>[2x]MNLKDSIGLRIKTERERQQMSREVLCLDGAELTVRQLIRIEKGESLPSLDRLSYIAKRLGKSMTELLDQDNITIPDEYYEMKNRLIKFPTYRNPDRIKSKLTLIEEVYEKFFDILPEEELLTLDILENILSFTSWEESPKVEEIYEDLFEQVKRKRKFSTNDLLVIDYYFFHLYGRKQYDKKLFERIIKRVLNQEIWTDDVYNIVLFNDLMAIAALKIFHNSFSDFLTVVDKALAVIEKSQLYSYKPSVFVLKAKYELLHKENKKEAAENYDKAIVFASVLEDSVLEESIKAGKLADGLGAGWSHPQFEK;>LPYFAGCL[2x]

Here, we elucidate the structure-function relationship of the transcription factor ComR, a new member of the RNPP family, which positively controls competence for natural DNA transformation in streptococci. ComR is directly activated by the binding of its associated pheromone XIP, the mature form of the comX/sigX-inducing-peptide ComS. XIP-binding induces release of the sequestered HTH domain and ComR dimerization to allow DNA binding. Each TPR domain is composed of 11 α-helices forming 5 TPR motifs followed by an additional C-terminal α-helix α16 called CAP.

The structure of the complex between full-length ComR from S. thermophilus LMD-9, the octapeptide XIP (ComS17-24 LPYFAGCL) and the pseudopalindromic 20 bp ComR-box from the comX promoter (5’-T10-A9-G8-T7-G6-A5-C4-A3-T2-A1.T1’-A2’-T3’-G4’-T5’-C6’-T7’-C8’-T9’-A10’-3’) has been determined at a resolution of 2.5 Å. The crystals diffracted in space group C2 with a dimer of the ComRS complex bound to one molecule of dsDNA per asymmetric unit. The two XRE-type HTH domains containing 5 α-helices (PROSITE documentation PDOC50943) interact with each other through loop α3-α4 and helix α5 whereas their two 32 Å-apart α3 helices perfectly accommodate in the successive DNA major groove of the two half-sites of the pseudopalindromic dsDNA fragment. H-bonds are made by two arginine residues from α3: R35 and R39. The interacting base pairs GC6, AT5, CG4 and AT3 of the ComR-box were previously shown to be essential for S. thermophilus ComR binding and form a highly conserved GACA motif in ComR-boxes of streptococci. The two TPR domains form a tight dimer characterized by an interface area of 978.5 Å2 and a calculated solvation free energy gain ΔiG of -6.2 kcal mol-1. In particular, salt bridges are formed between two pairs of interacting residues, K87-D200 and K246-E282. Helix α9 is broken and almost perpendicular to α8. Interestingly, the two DNA-binding domains display distinct relative orientations with their respective peptide-binding domain. The N-terminus of the peptide points toward the solvent whereas the C-terminus of the peptide is buried in a deep pocket, characterized by numerous hydrophobic interactions.> AVKYYTLEEIQKHNNSKSTWLILHYKVYDLTKFLEEHPGGEEV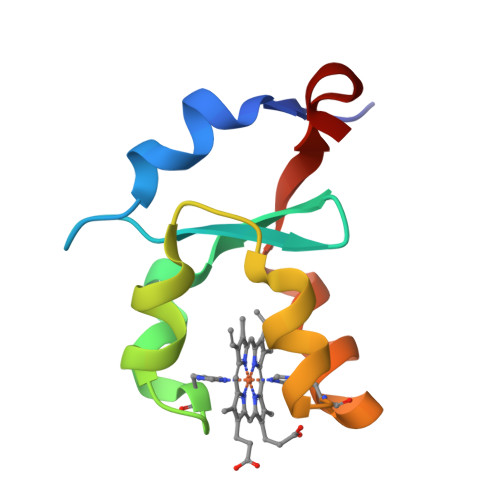LREQAGGDATENFEDHGHSTDARELSKTFIIGELHPDDR>TRDQNGTWEMESNENFEGWMKALDIDFATRKIAVRLTQTLVIDQDGDNFKVKSTSTFWNYDVDFTVGVEFDEYTKSLDNRHVKALVTWEGDVLVCVQKGEKENRGWKKWIEQDKLYLELTCGDQVCRQVFKKK[2x]

Human cellular retinol binding protein II (hCRBPII) was used as a protein engineering platform to rationally regulate absorptive and emissive properties of a covalently bound fluorogenic dye. We demonstrate the binding of a thio-dapoxyl analog via formation of a protonated imine between an active site lysine residue and the chromophore’s aldehyde. Previously, we showed the utility of human cellular retinol-binding protein II (hCRBPII) mutants as a fluorophoric tag, wherein an active site lysine residue (Q108K) reacts with synthetic aldehydic chromophores, giving rise to the formation of either an imine (Schiff base, SB) or an iminium (protonated SB, PSB). Q108K functions as the active-site lysine and forms a Schiff base with the aldehyde, whereas the K40L mutation is assumed to eliminate interactions between Q108K and Lys40, an interaction that could otherwise impede imine formation, and is also required to promote Schiff base protonation.

A conserved water network connecting the hydroxyl group of Tyr19 and the thiophene sulfur atom of TD-1V was observed in the M11 crystal structure. This observation marked Tyr19 as a residue for exchange into one that could disrupt this organized water network. Although incorporation of the Y19W mutation with R58H did not alter the spectroscopic characteristics of the protein/fluorophore complex (M13), surprisingly, when coupled with R58W, it led to a 30 and 22 nm red-shift in absorption and emission, respectively (M11 vs M14). Gratifyingly, the crystal structure of M14/TD-1V was obtained and showed that substitution of tryptophan for Tyr19 did indeed disrupt the water network observed in the M11/TD-1V crystal structure. The explanation for why only the combination of Y19W with R58W led to the significant change in spectral shift as opposed to the combination of R58H and Y19W is probably due to the nearly 90° rotation of the chromophore trajectory enforced by its interaction with Trp58 for M11. Exactly the same orientation is seen in the M14/TD-1V crystal structure, confirming the key and exclusive role Trp58 plays in causing the rotation of TD-1V in the binding pocket. For example, neither R58W nor Y19W are individual “winners”, but together they lead to a substantial effect. With the changes thus far, M14/TD-1V complex exhibits a bathochromic shift in absorption and emission (Δabs = 73 nm, Δem = 45 nm) relative to its parent mutant complex (M1/TD-1V).>[2x]MQVETWNAAELVAKDIAHHLHPLTN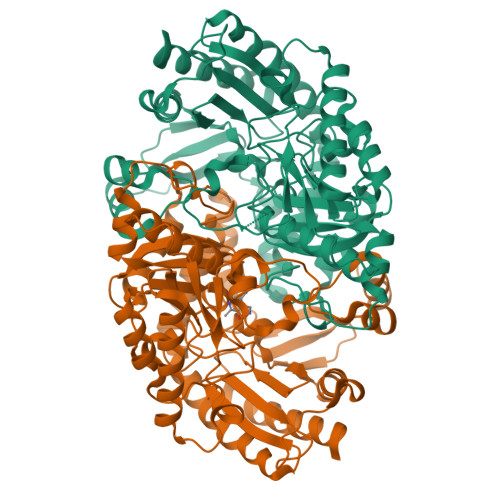LYQLRREGPLVLVRGEGVWVWDAEGKRYLDGFAGLWNVNIGHGRRELAEAAREQMERVAFVPTFFGLASPPTIELAARLAELFPGPLDHFQFTSGGAESNETAIKIARYYWWLKGQPERVKILSRRMAYHGIAMGALSATGVPAYWEGFGPRPPGFIHLTAPYKYRFGEGLTDEEFVARLVQELEETIEREGSETIAAFIGEPVQGAGGVVVPPDGYWPAIAAVLRKYGILLILDEVITGFGRTGTLFGMQQYGVQPDIVTFAKGITSGYVPLGGVGVSDEIAETLASADRVFMHGFTYSGHPVACAVALRNLDILLAERLWENAAASGAYLLQELKRLEERPYVGEVRGKGLMLLVEVVRDKASKEKFPPEFKLGPKLEAATRRRGIIVRCTPDGIVMAPPLTISRAECDVLIEGVAAALSDVLD(2R)-2-hydroxy-3-{[(S)-hydroxy{[(1S,2R,3R,4S,5S,6R)-2,3,4,5,6-pentahydroxycyclohexyl]oxy}phosphoryl]oxy}propyl 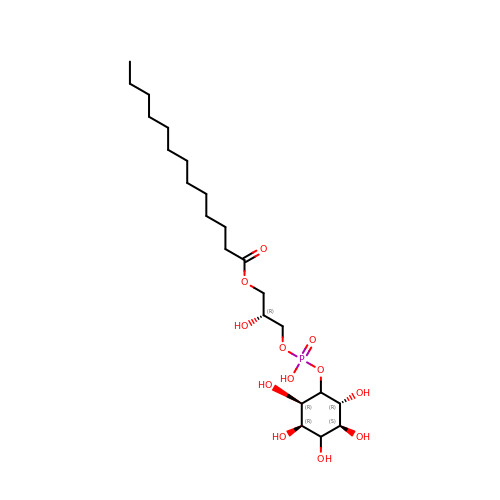tridecanoate | C22 H43 O12 P | QGSQXOJTKFYHRK-FBYKMOGESA-N>[2x]PVTTSFWRIATDARTYEA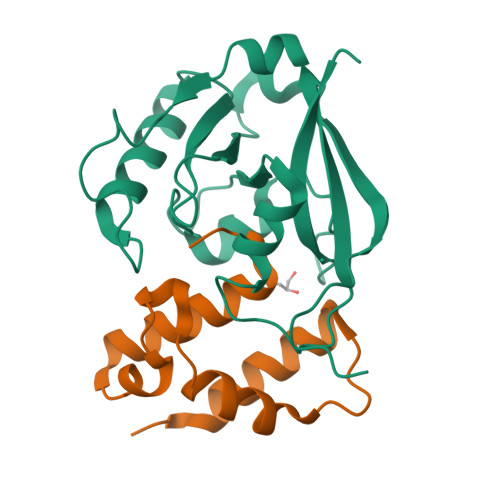DDLSGAGAKITGGRWNEVGVAIVYAASSRALACLETVVHLNSGGLPLNRYLVEIEVPDEVLASAEVATPGNLPVGWDAEPAGRVSISFGSQWAQSQRTALLLVPSVIVPEETNLLINPAHPDAKGIKARKVRKWLYDPRMIR;>VLGLAKLVGQLEDMVEESGETDGFDAPEWLSSWLRQPLPALGGVNPIDLLDTMEGQAVVSRALAQIQSGAFA[2x]>MITMKKIGVILSGCGVYDGSEIHEAVLTLLAISRSGAQAVCFAPDKQQVDVINHLTGEAMTETRNVLIEAARITRGEIRPLAQADAAELDALIVPGGFGAAKNLSNFASLGSECTVDRELKALAQAMHQAGKPLGFMCIAPA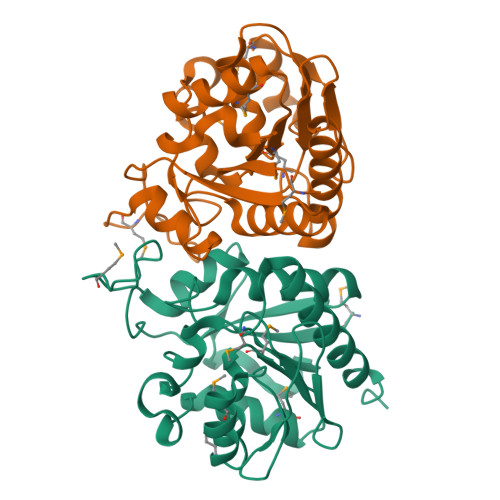MLPKIFDFPLRLTIGTDIDTAEVLEEMGAEHVPCPVDDIVVDEDNKIVTTPAYMLAQNIAEAASGIDKLVSRVLVLAELEHHHHHH[4x]>FTLIELAIVI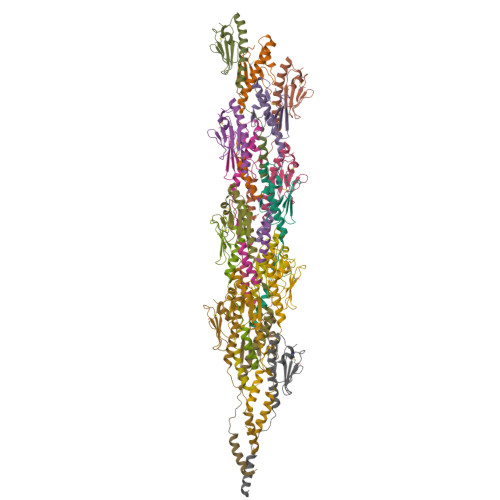VIIGILVAIAVPRFVDLTDQANQANVDATAAAVRSAYAIATVQAKGIPTCDQVFANPEGGSTSGSTWTSSDNSTTVSCNASADTFTISRGGKTRTLNLTVN[16x]>[5x]MESNLTTAASVIAAALAVGIGSIGPGLGQGQAAGQAVEGIARQPEAEGKIRGTLLL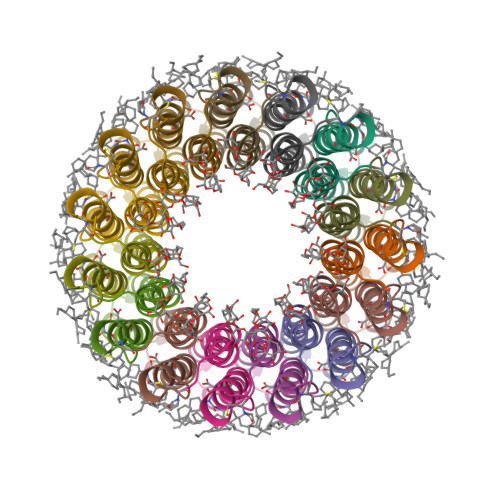SLAFMEALTIYGLVVALVLLFANPFV>[6x]MLNRIIEHMNAHHVEDMKGLLKKFGQVHHAENVAFKSVDSQGIVIGYNNNQTLRIEFNHEVKDPKDYKNATIELCQSVEKTHDLKGVEEEVKAFKEGFDSVCLATLHPNGHVVCS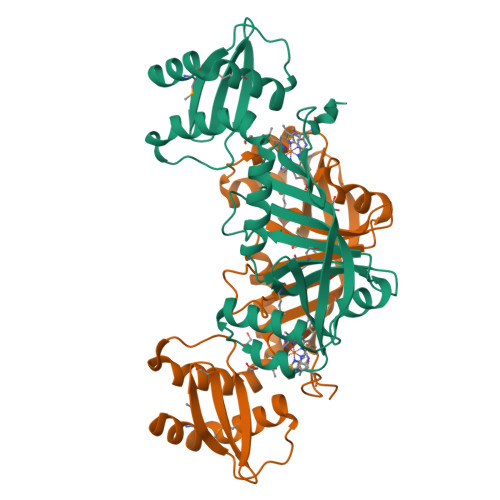YAPLMSDGKQYYIYVSEVAEHFAGLKNNPHNVEVMFLEDESKAKSAILRKRLRYKTNTRFIERGAEFDKAFDSFIEKTGGAGGIKTIRAMQDFHLIALDFKEGRFVKGFGQAYDILGDKIAYVGDKGNPHNFAHKKLEHHHHHH> PPSNPPPRPPAEARK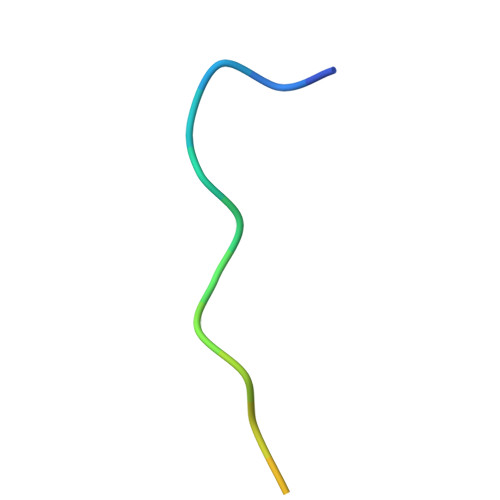KPS>[4x]MAASGEPQRQWQEEVAAVVVVGSCM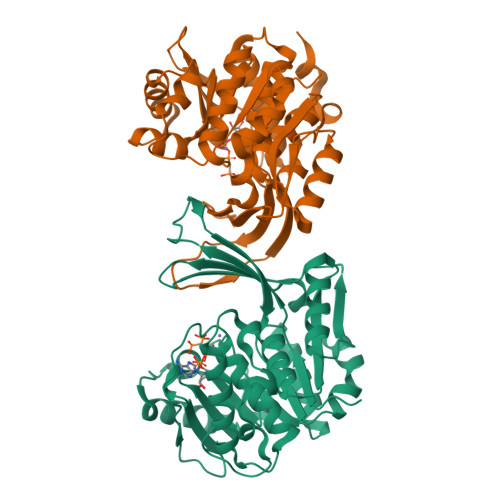TDLVSLTSRLPKTGETIHGHKFFIGFGGKGANQCVQAARLGAMTSMVCKVGKDSFGNDYIENLKQNDISTEFTYQTKDAATGTASIIVNNEGQNIIVIVAGANLLLNTEDLRAAANVISRAKVMVCQLEITPATSLEALTMARRSGVKTLFNPAPAIADLDPQFYTLSDVFCCNESEAEILTGLTVGSAADAGEAALVLLKRGCQVVIITLGAEGCVVLSQTEPEPKHIPTEKVKAVDTTGAGDSFVGALAFYLAYYPNLSLEDMLNRSNFIAAVSVQAAGTQSSYPYKKDLPLTLFLEHHHHHH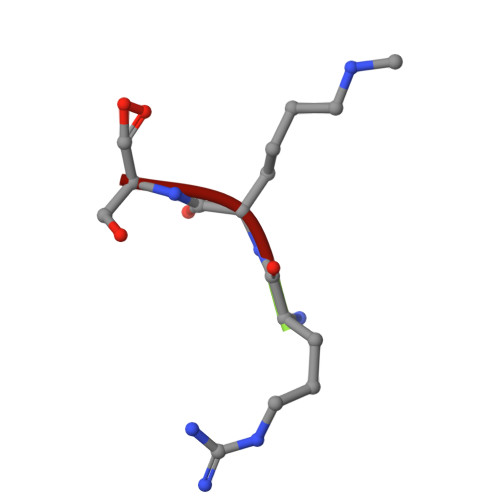> RKS Glutathione S-transferases are a family of detoxifying enzymes that catalyze the conjugation of reduced glutathione (GSH) with different xenobiotic compounds using either Ser, Tyr, or Cys as a primary catalytic residue. We identified a novel GST in the genome of the shrimp pathogen V. parahaemolyticus FIM- S1708+, a bacterial strain associated with Acute Hepatopancreatic Necrosis Disease (AHPND)/Early Mortality Syndrome (EMS) in cultured shrimp. This new GST class was named Gtt2.

The crystal of VpGSTT2 had a monoclinic unit cell with space group P1211, and the diffraction data of VpGSTT2-GTS were scaled and refined at a resolution of 1.92 Å. VpGSTT2 consists of two monomers per asymmetric unit. Each has the canonical GST topology, with a thioredoxin-like domain at the N-terminus and a globular C-terminal domain. The GSH-binding domain (residues 1–81) is called the G-site, while the hydrophobic substrates are bound at the H-site (residues 82–204). The RMSD between the two monomers in the asymmetric unit was 0.36 Å, with only minor differences in the N-terminal domain’s loops and β-sheet 2. VpGSTT2 crystallized only in the absence of ligands. Although VpGSTT2 is an apo structure, a crystallographic water molecule coordinated by the potential nucleophiles Thr 9 and Ser11 was observed. The electron density was clear for residue H2O-300 for monomer A and H2O-107 for monomer B. In the apo-VpGSTT2, a loop containing residues 36–39 moved towards the G-site cavity, causing steric hindrance to GSH binding. The double mutant lacked detectable activity, which led us to conclude that water was the general base catalyst.

>[2x]MKLYETAMTPSCKRVSIFLKEIGGEVERVALNVREGDNLSESFKQKSVNGKVPLLELDDGTTICESVAICRYLDEAFENDLALFGANQLERAQVEMWHRVVEFQGLYAAFQAFRNITAIYQDRENCVAAWGEESKSRVLEFLPTLDTRLSESEYIATDQFSVVDITGYIFIGFAVNGLSIEVFEKYPNIARWFEQVSARDAFQSSGLEVLFQ>GSHMGGYEIPARLRTLHNLVIQYASQGRYEVAVPLCKQALEDLEKTSGHDHPDVATMLNILALVYRDQNKYKDAANLLNDALAIREKTLGRDHPAVAATLNNLAVLYGKRGKYKEAEPLCKRALEIREKVLGKDHPDVAKQLNNLALLCQNQGKYEEVEYYYQRALGIYQTKLGPDDPNVAKTKNNLASCYLKQGKFKQAETLYKEILTRAHEREFGSVDDENKPIWMHAEEREECKGKQKDGSAFGEYGGWYKACKVDSPTVTTTLKNLGALYRRQGK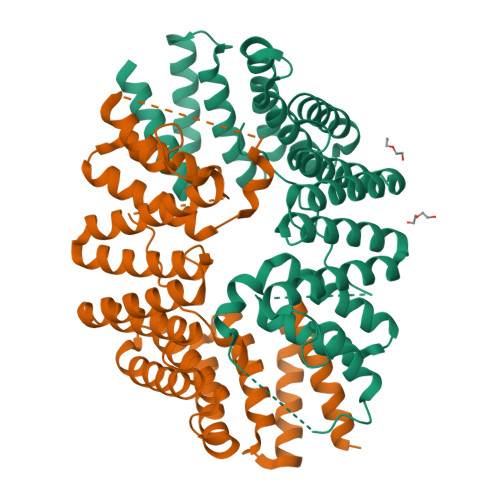FEAAETLEEAAMRSRKQTGSTGSTGSTGSTGSTGSTGSTGSTGSTGSGTVFTTEDIYEWDDSAI[6x]> MAAKGDMLYAWAKDAEIQKKGECGGAVTALLKHALETKMVDAVVAIKKGKDLYDAVPTVITNPEDIIQTAGSLHCGTLLIPKLIKKYLNGAKDMKLAVTCKGCDAMAFYELAKRNQIN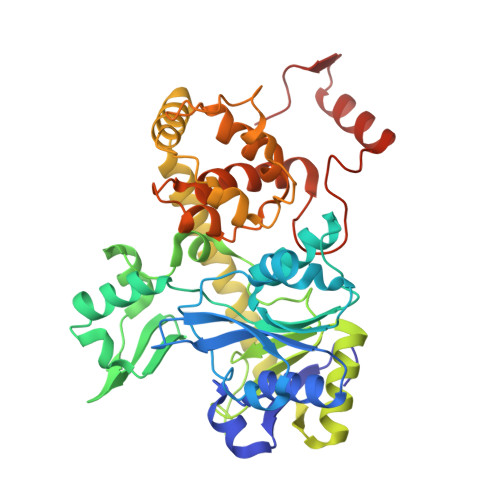LDNIIMIGVNCGGSVSPVTARKMISNKFGVDPDTVHKEEIDKGQFIIEYEGGHKGIKIDELEEEGYGRRSNCRRCKMKIPRQADIAAGNWGVIGDKAGKATFLEICSEKGANLVNSAQSKGALEISPADPKGIDIRAKVEKAMFNLGDEWRHRDFEGMGKGKDRLKLMMSESSKCIKCYACVEACPICYCIECSTKKPWYIAPGVLPTSFMFHLIRFAHVSDSCINCGQCEELCPMEIPNALFMHSQQVEIEKMFGHIPGQDMTPPIHAFVEEKAERARLDATGTDSIYTNIFTDE> MTWPLPDRLSINSLSGTPAVDLSSFTDFLRRQAPELLPASISGG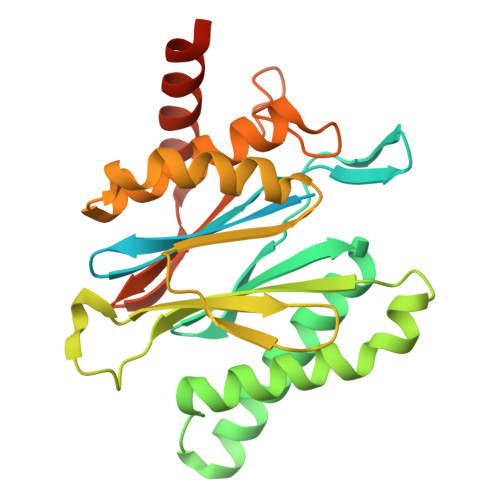APLAGGDAQLPHGTTIVALKYPGGVVMAGDRRSTQGNMISGRDVRKVYITDDYTATGIAGTAAVAVEFARLYAVELEHYEKLEGVPLTFAGKINRLAIMVRGNLAAAMQGLLALPLLAGYDIHASDPQSAGRIVSFDAAGGWNIEEEGYQAVGSGSLFAKSSMKKLYSQVTDGDSGLRVAVEALYDAADDDSATGGPDLVRGIFPTAVIIDADGAVDVPESRIAELARAIIESRSGADTFGSDGGEK>[2x]MDPYSETSDLVDISRFDTHGLGANYKLRRHKFEHLADTGCHKARSDWVKYIGPLTEFGGCNHINGNFSAVVLPLCRPDRLELIAYVLEFAFLHDSVLESENTSPESEVQAEAGLRLLYERCISRLLQTDEVCAKKIAKTWKDAINTTTKDKNVDFQSIEDYLEFRMIDTGAPFVEALMLFGLGMSLSPQEDDALGHVIRPCFAALALTNDYFSFDREIEEVDTSTLINSVAIVMRIQSLDIPTAKTIINETIQKYEREFLRRIDEYKQHKGPISNKIEQYMEAMTYQISGNLVWSLNCPRYNPDYRYGLEACQHEG

Here, we describe the discovery that class I terpene cyclases are bifunctional, in that they catalyze both terpene cyclization and aromatic prenyltransferase reactions in the same active site. Class I terpene cyclases require 3 Mg2+ ions for catalytic function, and these metal ions are coordinated by conserved metal-binding motifs in a unique α-helical protein fold. Interestingly, the diterpene synthase FgGS can accept GPP as substrate donor to produce long-chain prenylindoles 11–14. Compounds 11 and 14 were characterized as previously reported (E)-1-(3,7-dimethylocta-2,6-dien-1-yl)-1H-indole and (E)-3-(3,7-dimethylocta-2,6-dien-1-yl)-1H-indole, respectively. This characterization implies that the active site cavity of FgGS is sufficiently large to allow the binding of indole as well as C5 DMAPP or C10 GPP to produce prenylindoles.

To determine structure–function relationships in a second terpene cyclase with cryptic aromatic prenyltransferase activity, we determined the X-ray crystal structure of FgGS complexed with 3 Mg2+ ions, PPi, and the benzyltriethylammonium cation (BTAC) at 1.46 Å resolution. However, the second aspartate residue in the aspartate-rich motif of FgGS is substituted with serine, so this motif appears as D94SVLE98. Even so, metal coordination interactions are as expected: the side chain of D94 coordinates to Mg2+A and Mg2+C with syn–syn bidentate geometry, and Oδ2 of E98 coordinates to Mg2+A and Mg2+C with monodentate bridging geometry. Interestingly, Oδ1 of E98 coordinates to a Na+ ion outside of the enclosed active site cavity. The PPi anion is stabilized by hydrogen bonds with R165, T169, N209, R216, R300, and Y301. The BTAC cation binds in the lower cavity and its positively charged quaternary amino group engages in cation-π interactions with F67, F91, and W294. Additionally, the aromatic ring of BTAC makes a favorable edge-to-face interaction with F67. However, active site closure in FgGS also traps two ordered water molecules at the periphery of the lower active site cavity. Additionally, in the upper active site cavity there are two ordered waters (W21 and W22) and an ethylene glycol molecule (monomer A), or five ordered water molecules (W93, W101, W126, W222, and W263) and an ethylene glycol molecule (monomer B). The binding of the bulky BTAC molecule reveals that there is more than enough volume to accommodate the small 5-carbon prenyl group of DMAPP in the active site pocket.>GASMPLKPEEHEDILNKLLDPELAQSERTEALQQLRVNYGSFVSEYNDLTKSKMRRDLEEATLQHEATAAALRKKHADSVAELGEQIDNLQRVKQKLEKEKSEFKLELDDVTSNMEQIEKERDFYFGKLRNIELICQENEGENDPVLQRIVDILYATD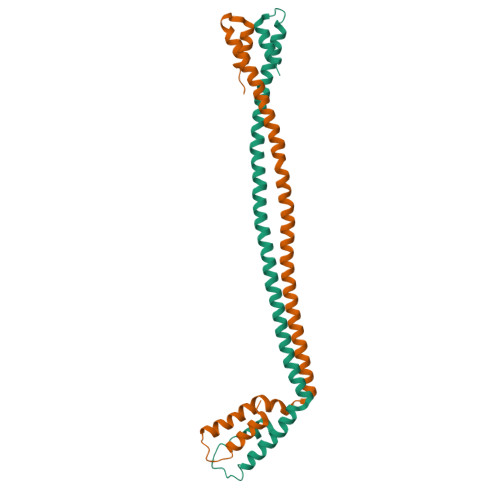E[4x]> SHMEAHLYMQVQIVAEDQFCGHQGNDMYDEEKVKYTVFKVLKNSSLAEFVQSLSQTMGFPQDQIRLWPMQARSNGTKRPAMLDNEADGNKTMIELSDNEN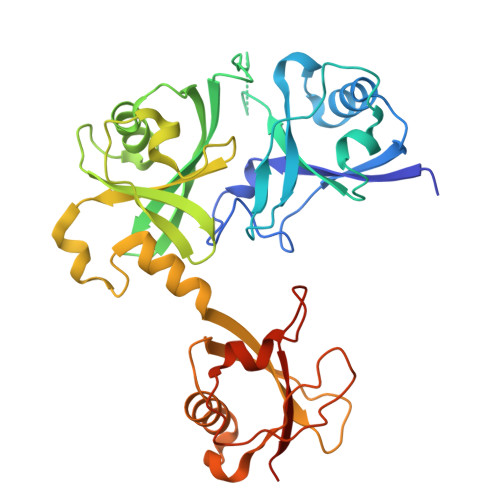PWTIFLETVDPELAASGATLPKFDKDHDVMLFLKMYDPKTRSLNYCGHIYTPISCKIRDLLPVMCDRAGFIQDTSLILYEEVKPNLTERIQDYDVSLDKALDELMDGDIIVFQKDDPENDNSELPTAKEYFRDLYHRVDVIFCDKTIPNDPGFVVTLSNRMNYFQVAKTVAQRLNTDPMLLQFFKSQGYRDGPGNPLRHNYEGTLRDLLQFFKPRQPKKLYYQQLKMKITDFEN>GAIIFSAKDIFEQEFGREVRGYNKVEVDEFLDDVIKDYETYAALVKSLRQ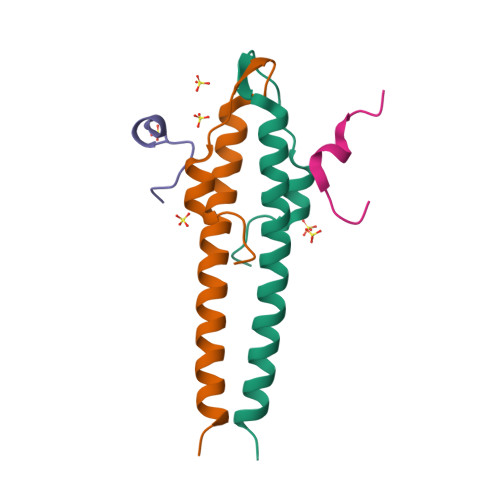EIADLKEELTRK[2x];>[2x]TILRRSRSDRKKLA> GQESCGPNEVWTECTGCEMKCGPDENTPCPLMCRRPS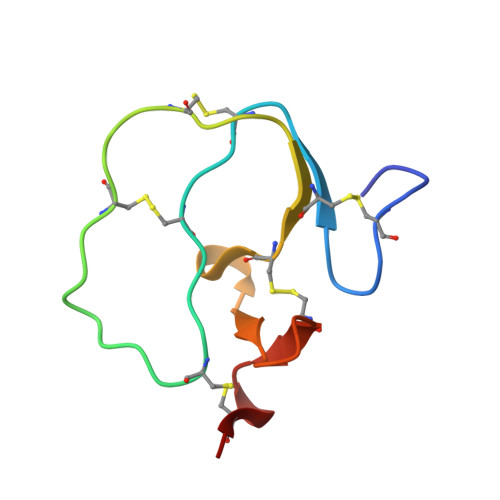CECSPGRGMRRTNDGKCIPASQCP2-[(cyclopropylcarbonyl)oxy]-3-methylbenzoic acid | C12 H12 O4 | 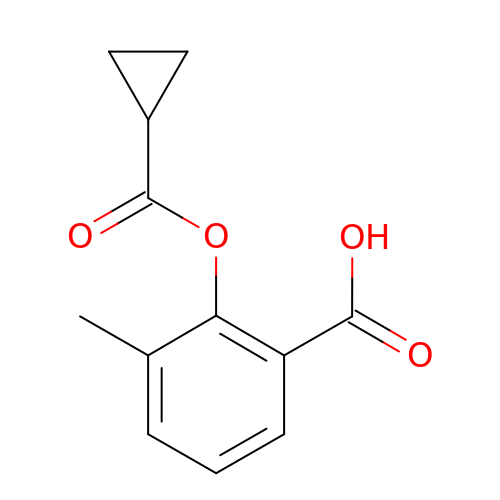RHIRFUJRCDAPMZ-UHFFFAOYSA-N2-(hydroxymethyl)-6-methoxy-phenol | C8 H10 O3 | 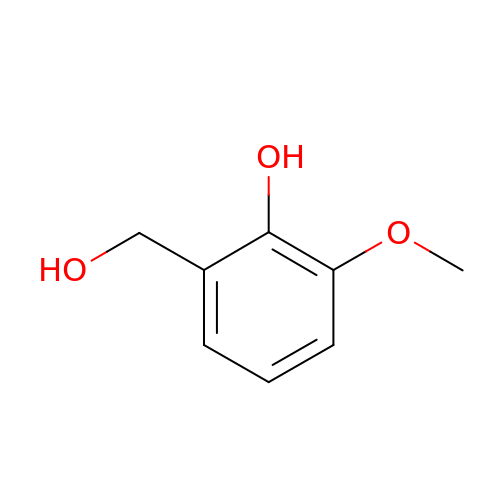OSZHSESNQIMXMZ-UHFFFAOYSA-N>[6x]GSGMSYTMCSGKFSIDK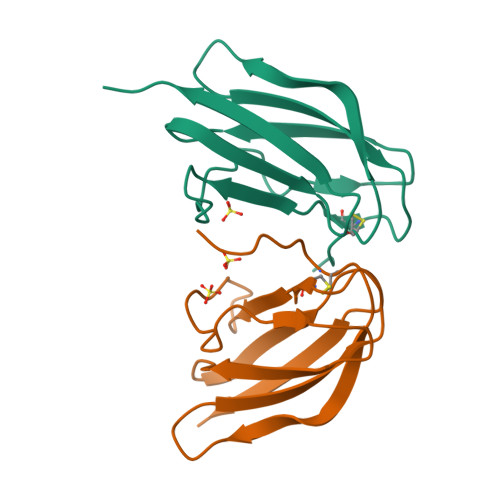EMAETQHGTTVVKVKYEGAGAPCKVPIEIRDVNKEKVVGRIISSTPLAENTNSVTNIELEPPFGDSYIVIGVGDKALKLNWFRKGSSIGK> PKPWLGAQPATVVTPGVNVTLRCRAPQPAWRFGLFKPGEIAPLLFRDVSSELAEFFLEEVTPAQGGIYRCCYRRPDWGPGVWSQPSDVLELLVTEELPRPSLVALPGPVVGPGANVSLRCAGRLRNMSFVLYREGVAAPLQYRHSAQPWADFTLLGARAPGTYSCYYHTPSAPYVLSQRSEVLVI;>GPPGPPG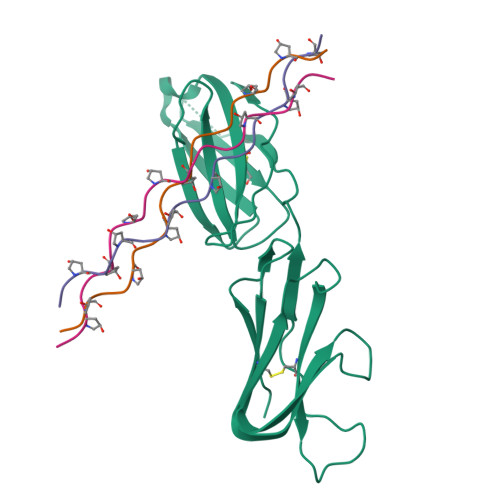PPGPPGPAGFPGPPGPPG[3x]> GIDPFTSTQQHTEPAEEETLHNIITDTENVQGSFSKHEFQAETKKLLDIVARSLYSEKEVFIRELISNGSDALEKLRHRMITAGGDTAPMEIHLQTDSVKGTFTIQDTGVGMNKEDLVSNLGTIARSGSKAFLDALQNQAEASSSIIGQFGVGFYSAFMVADKVEVYSQSAEADAPGYKWSSDGSGVFEVAEASGVRQ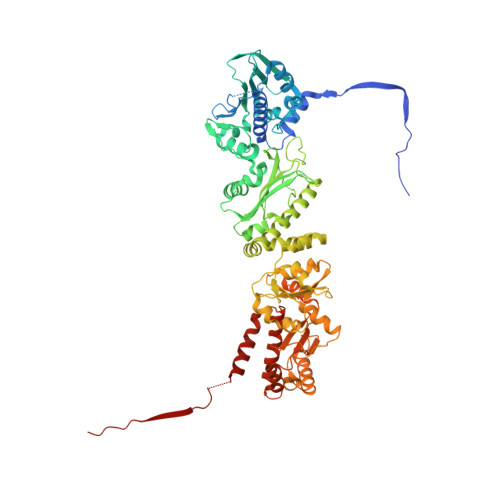GTKIVLHLKDDCKEFSSEDRVKEVVTKYSNFVSFPIFLNGRRLNTLQALWMMEPKDISEWQHEEFYRYVAQAYDKPRYTLHYRADAPLNIRSIFYVPEMKPSMFDVSREMGSSVALYSRKILIQTKATDILPKWLRFLRGVVDSEDIPLNLSAELLQESALIRKLRDVLQQRVIRFLLDQSKKDPEKYARFFEDYGLFMREGIVTTGEQSVKEDIAKLLRFESSALPAGQQTSLMEYSSRMKAGTRNIYYLCAPNRHLAEHSPYFEAMKQKDMEVLFCFEQFDELTLLHLREFDRKKLISAETDIVVDHYKEEKFQDSKPASERLSSEQAEDLLAWMRNALVQRVTNIKVTPRLDTHPAMITVLEMGAARHFLRTQQLARSSEERAQILQPTLEINTGHDLIKKLHALKDSNPELAQLLLEQIYDNAMIAAGLNEDPRPMISRLNQLLTRALEKHGGSGSSAHIVMVDAYKPTK> MSESQTLDKVYQMKSKPRGYCLIINNHNFAKAREKVPKLHSIRDRNGT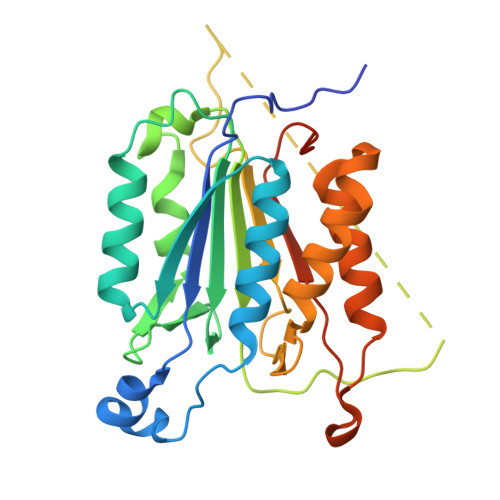HLDAGALTTTFEELHFEIKPHDDCTVEQIYEILKIYQLMDHSNMDCFICCILSHGDKGIIYGTDGQEAPIYELTSQFTGLKCPSLAGKPKVFFIQACQGDNYQKGIPVETDSEEQPYLEMDLSSPQTRYIPDEADFLLGMATVNNCVSYRNPAEGTWYIQSLCQSLRERCPRGDDILTILTEVNYEVSNKDDKKNMGKQMPQPTFTLRKKLVFPSDAAALEHHHHHH> GAMTIRHQGQQYRPRMAFLQKIEALVKDMQNPETGVRMHNQRVLVTSVPHAMTGGDVLQWITQRLWISNLEAQNLGNFIVKYGYIYPLQDPKNLILKPDSSLYRFQTPYFWPTQQWPAEDTDYAIYLAKRNIKKKGILEEYEKENYDFLNKKINYKWDFVIMQAKEQYRTGKERNKADRYALDCQEKAYWLVHRSPPGMNNVLDYGLDRVTNPNEVKKQTVTAVRKEIMYYQQALMRSTVKSSVSLGGIVKYSEQFSSNDAIMSGCLPSNPWITDDTQFWDLNAKLVEIPTKMRVERWAFNFSELIRDPKGRQSFQYFLKKEF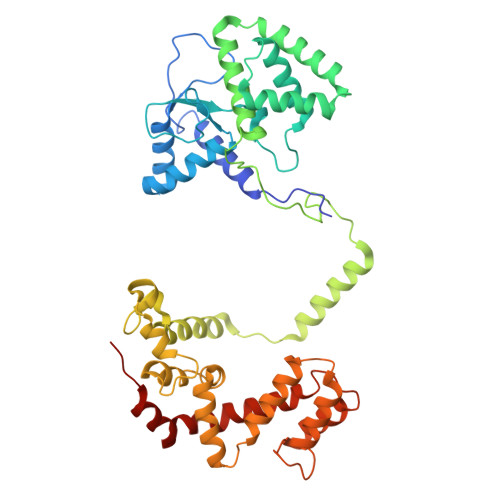SGENLGFWEACEDLKYGDQSKVKEKAEEIYKLFLAPGARRWINIDGKTMDITVKGLRHPHRYVLDAAQTHIYMLMKKDSYARYLKSPIYKEMLAKAIEPQE>MRMRHKPWADDFLAENADIAISNPADYKGKWNTVFGNDNPIHIEVGTGKGQFISGMAKQNPDINYIGIELFKSVIVTAVQKVKDSEAQNVKLLNIDADTLTDVFEPGEVKRVYLNFSDPWPKKRHEKRR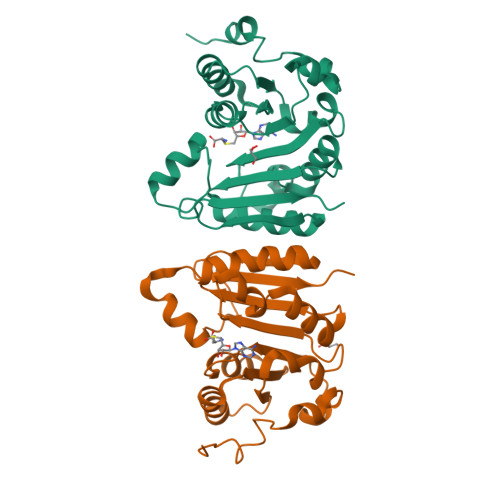LTYSHFLKKYEEVMGKGGSIHFKTDNRGLFEYSLKSFSEYGLLLTYVSLDLHNSNLEGNIMTEYEEKFSALGQPIYRAEVEWRT[2x]>HPETLVKVKDAEDQLGARVGYIELDLNSGKILESFRPEERFPMMSTFKVLLCGAVLSRVDAGQEQLGRRIHYSQNDLVEYSPVTEKHLTDGMTVRELCSAAITMSDNTAANLLLTTIGGPKELTAFLHNMGDHVTRLDRWEPELNEAIPNDERDTTNPAAMATTLRKLLTGELLTLASRQQLIDWMEADKVAGPLLRS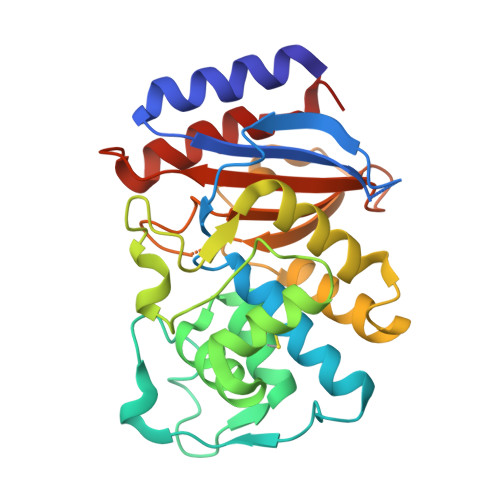ALPAGWFIADKSGAGERGSRGIIAALGPDGKPSRIVVIYTTGSQATMDERNRQIAEIGASLIKHW[4x]> SMPRVDFPRSRLRFKEKLGEGQFGEVHLCEVDSPQDLVSLDFPLNVRKGHPLLVAVKILRPDATKNARNDFLKEVKIMSRLKD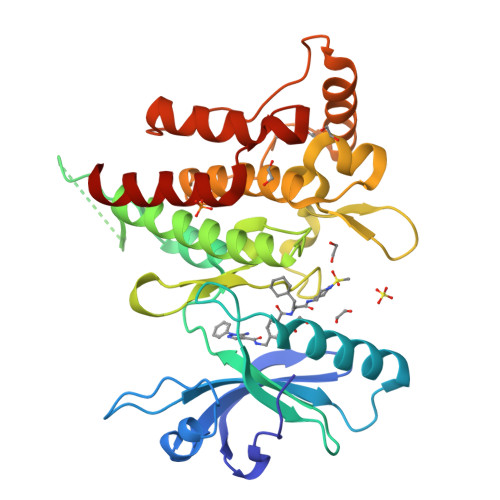PNIIRLLGVCVQDDPLCMITDYMENGDLNQFLSAHQLEDKAAEGAPGDGQAAQGPTISYPMLLHVAAQIASGMRYLATLNFVHRDLATRNCLVGENFTIKIADFGMSRNLYAGDYYRVQGRAVLPIRWMAWECILMGKFTTASDVWAFGVTLWEVLMLCRAQPFGQLTDEQVIENAGEFFRDQGRQVYLSRPPACPQGLYELMLRCWSRESEQRPPFSQLHRFLAEDALNTV>[2x]MGSYLSSLLGGGAAEAAEAESGSSSEPSRVIAFHSSNRWQLHFNSSKQLNKLIVVDFAATWCGPCKMMEPVINAMSAKYTDVDFVKIDVDELSDVAQEFG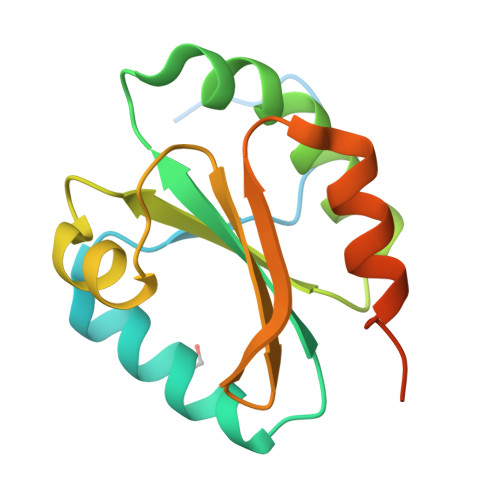VQAMPTFLLLKQGKEVERVVGAKKDELEKKILKHREAPKFAASNYRTKFHVQ> MNLLIDNWIPVRPRNGGKVQIINLQSLYCSRDQWRLSLPRDDMELAALALLVCIGQIIAPAKDDVEFRHRIMNPLTEDEFQQLIAPWIDMFYLNHAEHPFMQTKGVKANDVTPMEKLLAGVSGATNCAFVNQPGQGEALCGGCTAIALFNQANQAPGFGGGFKSGLRGGTPVTTFVRGIDLRSTVLLNVLTLPRLQKQFPNESHTENQPTWIKPIKSNESIPASSIGFVRGLFWQPAHIELCDPIGIGKCSCCGQESNLRYTGFLKEKFTFTVNGLWPHPHSPCLVTVKKGEVEEKFLAFTTSAPSWTQISRVVVDKIIQNENGNRVAAVVNQFRNIAPQSPLELIMGGYRNNQASILERRHDVLMFNQGWQQYGNVINEIVTVGLGYKTALRKALYTFAEGFKNKDFKGAGVSVHETAERHFYRQSELLIPDVLANVNFSQADEVIADLRDKLHQLCEMLFNQSVAPYAHHPKLISTLALARATLYKHLRELKPQGGPSNG;>[2x]MASHHHHHHGALEVLFQGPGYQMADEIDAMALYRAWQQLDNGSCAQIRRVSEPDELRDIPAFYRLVQPFGWENPRHQQALLRMVFCLSAGKNVIRHQDKKSEQTTGISLGRALANSGRINERRIFQLIRADRTADMVQLRRLLTHAEPVLDWPLMARMLTWWGKRERQQLLEDFVLTTNKNA;>MSNFINIHVLISHSPSCLNRDDMNMQKDAIFGGKRRVRISSQSL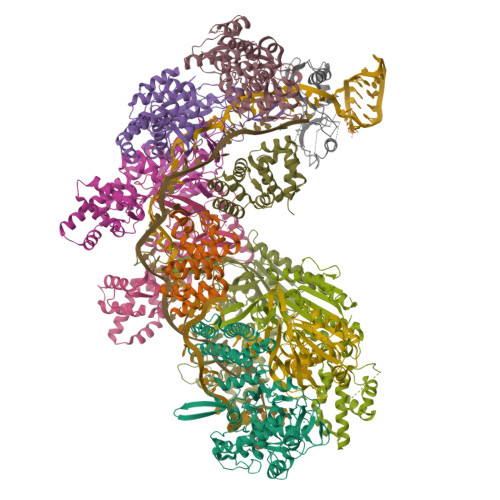KRAMRKSGYYAQNIGESSLRTIHLAQLRDVLRQKLGERFDQKIIDKTLALLSGKSVDEAEKISADAVTPWVVGEIAWFCEQVAKAEADNLDDKKLLKVLKEDIAAIRVNLQQGVDIALSGRMATSGMMTELGKVDGAMSIAHAITTHQVDSDIDWFTAVDDLQEQGSAHLGTQEFSSGVFYRYANINLAQLQENLGGASREQALEIATHVVHMLATEVPGAKQRTYAAFNPADMVMVNFSDMPLSMANAFEKAVKAKDGFLQPSIQAFNQYWDRVANGYGLNGAAAQFSLSDVDPITAQVKQMPTLEQLKSWVRNNGEA[6x];> MRSYLILRLAGPMQAWGQPTFEGTRPTGRFPTRSGLLGLLGACLGIQRDDTSSLQALSESVQFAVRCDELILDDRRVSVTGLRDYHTVLGAREDYRGLKSHETIQTWREYLCDASFTVALWLTPHATMVISELEKAVLKPRYTPYLGRRSCPLTHPLFLGTCQASDPQKALLNYEPVGGDIYSEESVTGHHLKFTARDEPMITLPRQFASREWYVIKGGMDVSQ;> MYLSKVIIARAWSRDLYQLHQGLWHLFPNRPDAARDFLFHVEKRNTPEGCHVLLQSAQMPVSTAVATVIKTKQVEFQLQVGVPLYFRLRANPIKTILDNQKRLDSKGNIKRCRVPLIKEAEQIAWLQRKLGNAARVEDVHPISERPQYFSGDGKSGKIQTVCFEGVLTINDAPALIDLVQQGIGPAKSMGCGLLSLAPL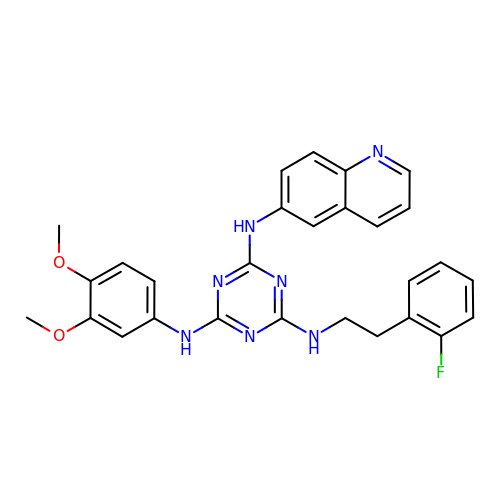N~2~-(3,4-dimethoxyphenyl)-N~4~-[2-(2-fluorophenyl)ethyl]-N~6~-quinolin-6-yl-1,3,5-triazine-2,4,6-triamine | C28 H26 F N7 O2 | FLCQZZIDGSESAD-UHFFFAOYSA-N> GGAAAATTTGG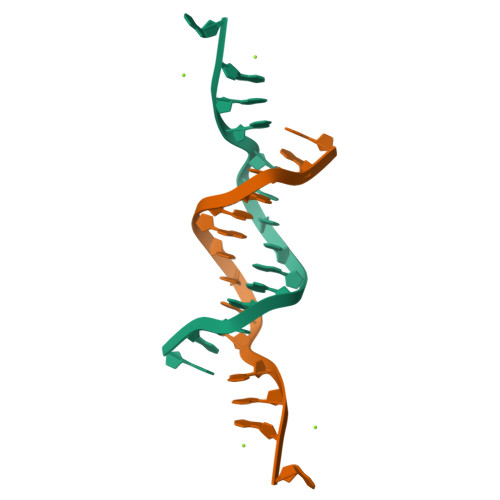AGA2-ethoxy-8-(5-fluoranylpyridin-3-yl)-9-[[4-[[(1S,4S)-5-methyl-2,5-diazabicyclo[2.2.1]heptan-2-yl]methyl]phenyl]methyl]purin-6-amine 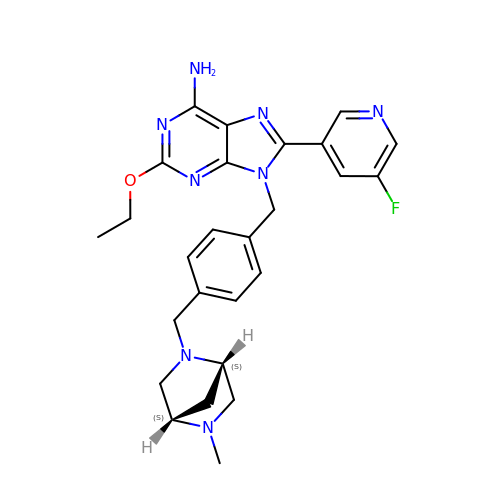| C26 H29 F N8 O | NHZSWKDFGUWVJJ-SFTDATJTSA-N> GMKLLLTRPEGKNAAMASALDALAIPYLVEPLLSVEAAAVTQAQLDELSRADILIFISTSAVSFATPWLKDQWPKATY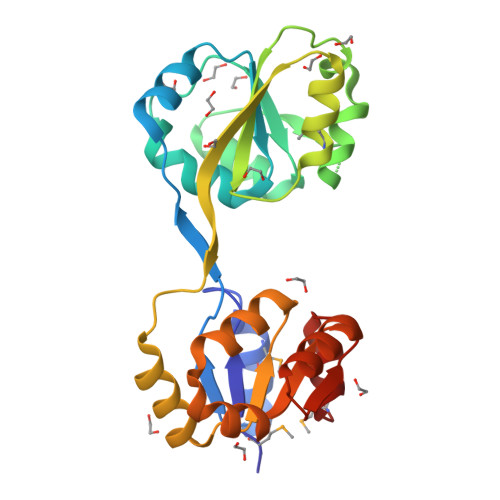YAVGDATADALALQGITAERSPADSQATEGLLTLPSLEQVSGKQIVIVRGKGGREAMADGLRLRGANVSYLEVYQRACPPLDAPASVSRWQSFGIDTIVVTSGEVLENLINLVPKDSFAWLRDCHIIVPSARVETQARKKGLRRVTNAGAANQAAVLDALGM> HPETLVKVKDAEDQLGARVGYIELDLNSGKILESFRPEERFPMMSTFKVLLCGAVLSRVDAGQEQLGRRIHYSQNDLVKYSPVTEKHLTDGMTVRELCSAAITMSDNTAANLLLTTIGGPKELTAFLHNMGDHVTRLDSWEPELNEAIPNDERDTTTPAAMATTLRKLLTGELLTLASRQQLIDWMEADKVAGPLLRSALPAGWFIADKSGAGERGSRGII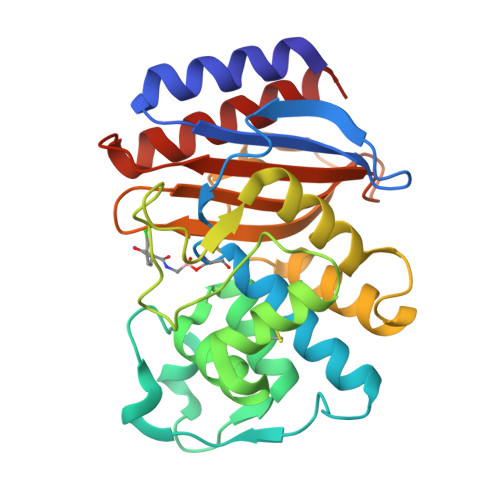AALGPDGKPSRIVVIYTTGSQATMDERNRQIAEIGASLIKHW> AGTGVVSVQ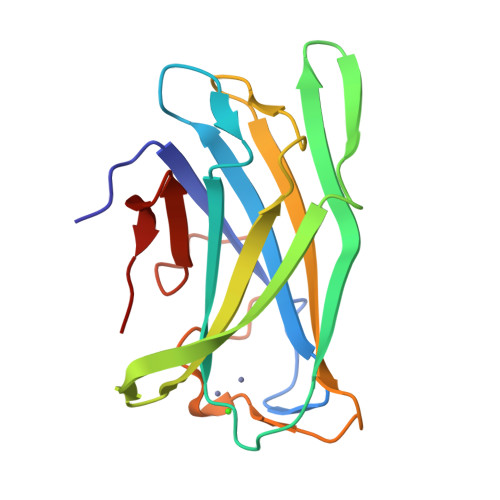FNNGSSPASSNSIYARFKVTNTSGSPINLADLKLRYYYTQDADKPLTFWCDHAGYMSGSNYIDATSKVTGSFKAVSPAVTNADHYLEVALNSDAGSLPAGGSIEIQTRFARNDWSNFDQSNDWSYTAAGSYMDWQKISAFVGGTLAYGSTP> MTGANVTFKVKGTDKEFTVFTTRPDTLFGATFTVLAPEHELVDAITSSEQ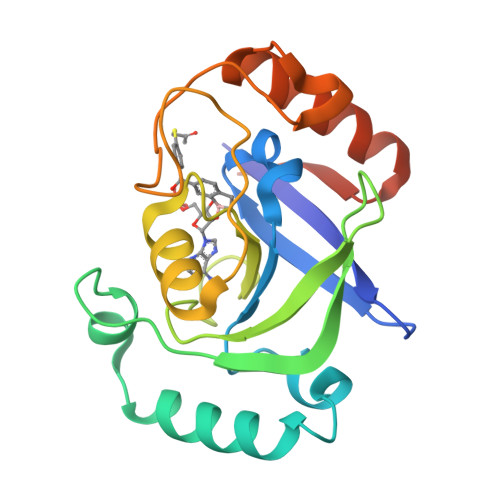AEAVADYKHQASLKSDLVRTDLAKEKTGVWTGAYAINPVNGKEMPIWIADYVLASYGTGAVMAVPAHDQRDWEFAKQFDLPIVEVLEGGNVEEAAYTEDGLHVNSDFLDGLNKEDAIAKIVASLEEKGCGQEKVLEHHHHHH> MATLRRLREAPRHLLVCEKSNFGNHKSRHRHLVQTHYYNYRVSFLIPECGILSEELKNLVMNTGPYYFVKNLPLHELITPEFISTFIKKGSCYALTYNTHIDEDNTVALLPNGKLILSLDKDTYEETGLQGHPSQFSGRKIMKFIVSIDLMELSLNLDSKKYERISWSFKEKKPLKFDFLLAWHKTGSEESTMMSYFSKYQIQEHQPKVALSTLRDLQCPVLQSSELEGTPEVSCRALELFDWLGAVFSNVDLNNEPNNFISTYCCPEPSTVVAKAYLCTITGFILPEKICLLLEHLCHYFDEPKLAPWVTLSVQGFADSPVSWEKNEHGFRKGG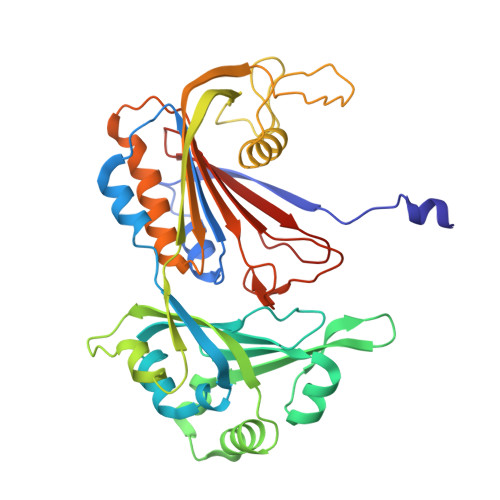EHLYNFVIFNNQDYWLQMAVGANDHCPP> GPLGSLTMGAQDTLPVAAAFTETVNAYFKGADPSKCIVKITGE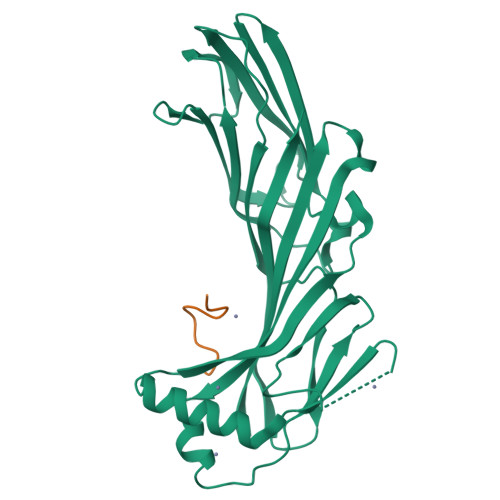MVLSFPAGITRHFANNPSPAALTFRVINFSRLEHVLPNPQLLCCDNTQNDANTKEFWVNMPNLMTHLKKVSEQKPQATYYNVDMLKYQVSAQGIQSTPLNLAVNWRCEPSSTDLRIDYKYNTDAMTTAVALNNVQFLVPIDGGVTKLQAVLPPAVWNAEQQRILWKIPDISQKSENGGVGSLLARFQLSEGPSKPSPLVVQFTSEGSTLSGCDIELVGAGYRFSLIKKRFAAGKYLADN;> YDPFKGSDPFA(4~{R})-4-[(3~{R},4~{R},5~{S},6~{R},7~{R},8~{S},9~{S},10~{R},13~{R},14~{R},17~{R})-6-ethyl-4-fluoranyl-10,13-dimethyl-3,7-bis(oxidanyl)-2,3,4,5,6,7,8,9,11,12,14,15,16,17-tetradecahydro-1~{H}-cyclopenta[a]phenanthren-17-yl]-~{N}-[4-(trifluoromethyloxy)phenyl]sulfonyl-pentanamide 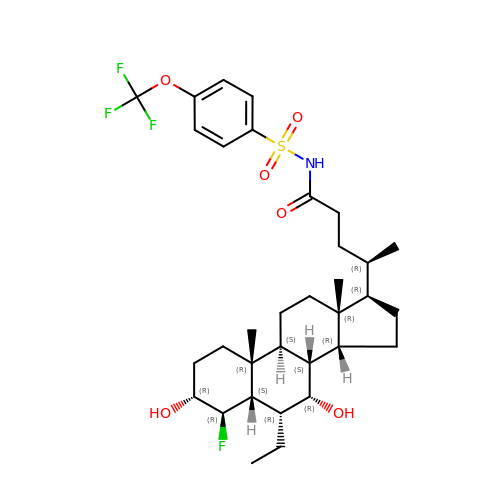| C33 H47 F4 N O6 S | ZGYUTSLXPGLWLX-KRYZBPAKSA-N> GRKRRQTSMTDFFHSKR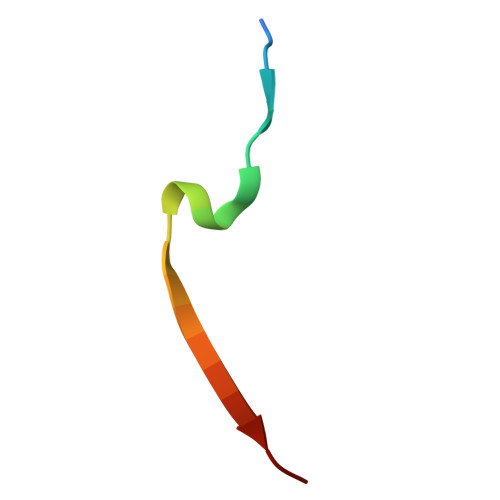RLIFS> GMNQSIIFTEQLTWDVQL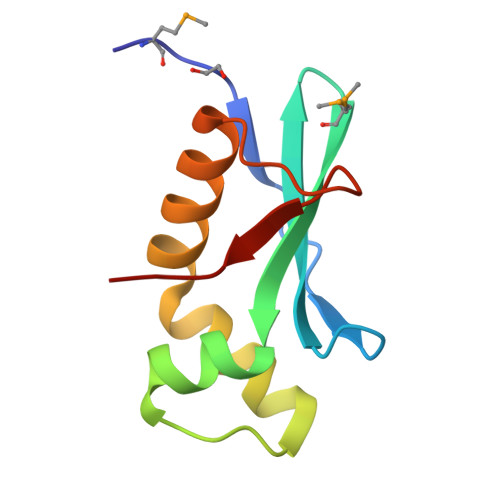SAIHFTAQQQGMVIDCYIGQKVLEHLAAEKINNSEQALSLFEQFRFDIEEQAEKLIEQEAFDVQGHIQVERVD>[12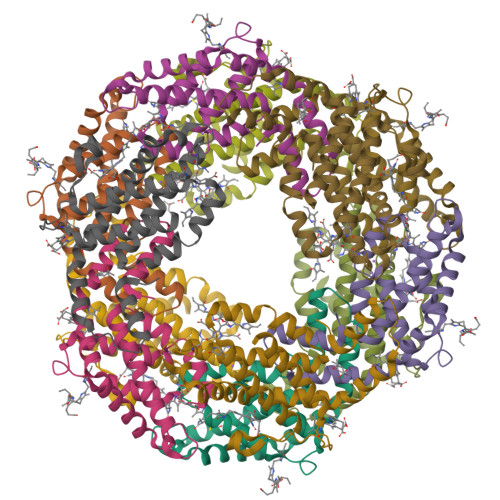x]MKSVVTTVIAAADAAGRFPSSSDLESVQGSIQRSAARLEAAEKLAGNIDAVAQEAYNACIQKYPYLNNSGEANSTDTFKAKCLRDVKHYMRLIQYSLVVGGTGPLDEWGIAGQREVYRALGLPTAPYVEALSFARNRGCAPRDMSAQALTEYNALLDYAINSLS;>[12x]MLDAFSRAVVQADASTSVVADMGALKQFIAEGNRRLDAVNAIASNASCMVSDAVAGMICENQGLIQAGGNCYPNRRMAACLRDAEIILRYVTYALLAGDASVLDDRCLNGLKETYAALGVPTTSTVRAVQIMKAQAAAHIKDTPSEARAGGKLRKMGSPVVEDRCASLVAEASSYFDRVISALS> MGSSHHHHHHSSGLVPRGSHHEATVHPERFEPLLERSVPRIQPGLSAVRELLTHQPAFDALERFSEDLLLCIFQDM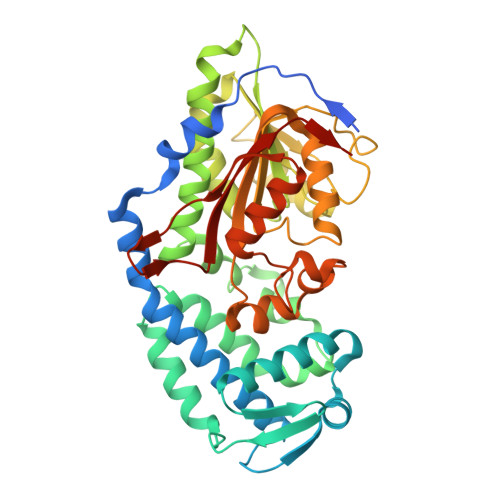GAFQRAGSAESAATLRERLGVAGRFGRLYDSLLAILEGAGYLRIEGDRLFTSERVTPKKHEVERRMQQLADLPAIAPYVRLLWACYRRYPELLRGQVAATDVLFPQGSMDLMGPLYKGNATADHFNELVIKSLLVFLDARVPHLREGEKITILEVGAGTGGTTASVLEALSSHARHLEYFYTDISHAFTRYGKRQYGPRYPFVTFQPLDLEGDVVAQGFSAERFDVVLGANVVHATKNLRSTLQSIKRLLKANGWLVLNEMTRVVHFLTLSAGLLDGWWLFEDAAERMKWSPLLSSPMWKGLLEEEGFRRVAPLQHSDGTSSWSIQNVILAESDGVSRSRRTESAA> GPGSCPTHADSLNNLANIKREQGNIEEAVRLYRKALEVFPEFAAAHSNLASVLQQQGKLQEALMHYKEAIRISPTFADAYSNMGNTLKEMQDVQGALQCYTRAIQINPAFADAHSNLASIHKDSGNIPEAIASYRTALKLKPDFPDAYCNLAHCLQIVCDWTDYDERMKKLVSIVADQLEKNRLPSVHPHHSMLYPLSHGFRKAIAERHGNLCLDKINVLHKPPYEHPKDLKLSDGRLRVGYVSSDFGNHPTSHLMQSIPGMHNPDKFEVFCYALSPDDGTNFRVKVMAEANHFIDLSQIPCNGKAADRIHQDGIHILVNMNGYTKGARNELFALRPAPIQAMWLGYPGTSGALFMDYIITDQETSPAEVAEQYSEKLAYMPHTFFIGDHANMFPHLKKKAVIDFKSNGHIYDNRIVLNGIDLKAFLDSLPDVKIVKMKCPDGGDNADSSNTALNMPVIPMNTIAEAVIEMINRGQIQITINGFSISNGLATTQINNKAATGEEVPRTIIVTTRSQYGLPEDAIVYCNFNQLYKIDPSTLQMWANILKRVPNSVLWLLRFPAVG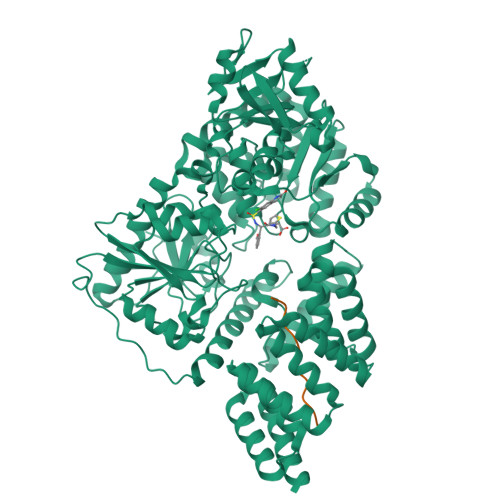EPNIQQYAQNMGLPQNRIIFSPVAPKEEHVRRGQLADVCLDTPLCNGHTTGMDVLWAGTPMVTMPGETLASRVAASQLTCLGCLELIAKNRQEYEDIAVKLGTDLEYLKKVRGKVWKQRISSPLFNTKQYTMELERLYLQMWEHYAAGNKPDHMIKPVE;> THETGTTNTATTATSN The 16S microbial community profiling of a metagenomics library from geothermal spring at Lisvori (Lesvos island, Greece) enabled the identification of a putative sequence exhibiting 95% identity to the γ‐type carbonic anhydrase (γ‐CA) from Caloramator australicus (γ‐CaCA). The sequence of γ‐CaCA was amplified by PCR, cloned, and expressed in E. coli. X‐ray crystallographic analysis of the γ‐CaCAmut structure at 2.1 Å resolution, provided detailed structural insights into how the mutations impact the overall enzyme structure, function, and thermostability. These findings provide valuable structural and functional insights into γ‐CAs and demonstrate a strategy for converting an inactive enzyme into a catalytically active form through rational design.

Structure‐based rational design enabled the design and creation of a mutant enzyme (γ‐CaCAmut) which possessed a heptapeptide insertion at the active‐site loop and two‐point mutations. Kinetic analysis demonstrated that γ‐CaCAmut was successfully converted into a catalytically active esterase indicating successful activity gain through structure‐guided engineering. The thermostability of γ‐CaCAmut was significantly increased, aligning with the thermostability typically observed in hyperthermostable enzymes.

>[9x]MEHKYKNHLPKIHETTFVAEGVHIIGDVEIGEDSNIWFNAVLRGDENSIKIGRGTNIQDNATLHASEVYHEEEIEQSPTIIGDYVTVGHNCIIHGCKIGDYSLIGMGSIILDNAEIGEYTIIGAGSLVTQNKKIPPRVLCMGSPAKVIRELTEEEIEYLKNSAKHNIELSKNYRHHHHHH;> WVAVWGDR> MTENGRYEYIVIGSEAAGVGLVRELTAAGKKVLAVDKSKEKIELLEDEGFDAVIADPTDESFYRSLDLEGVSAVLITGSDD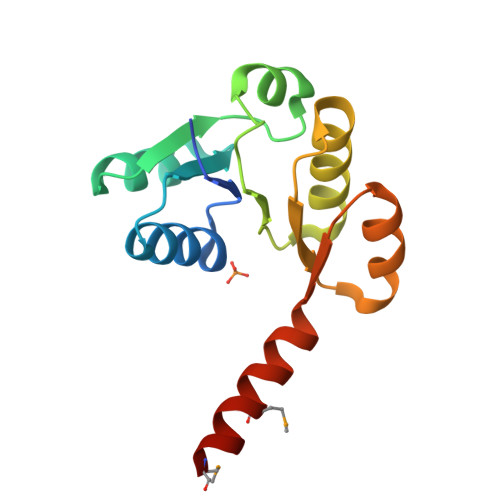EFNLKILKALRSVSDVYAIVRVSSPKKKEEFEEAGANLVVLVADAVKQAFMDKIKKMETL> GPGSEFPSQPKSVEDLLDRINLKEHMPTFL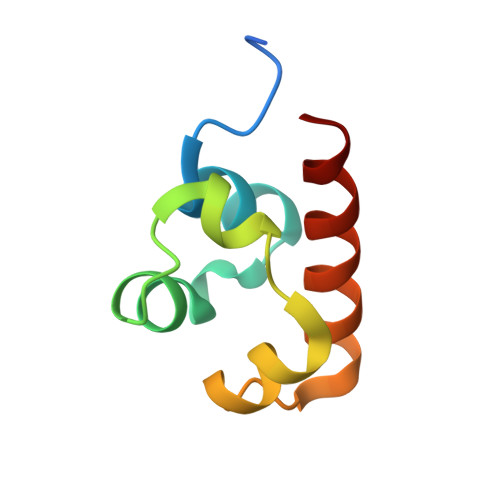FNGYEDLDTFKLLEEEDLDELNIRDPEHRAVLLTAVELLQEYD>[2x]MLI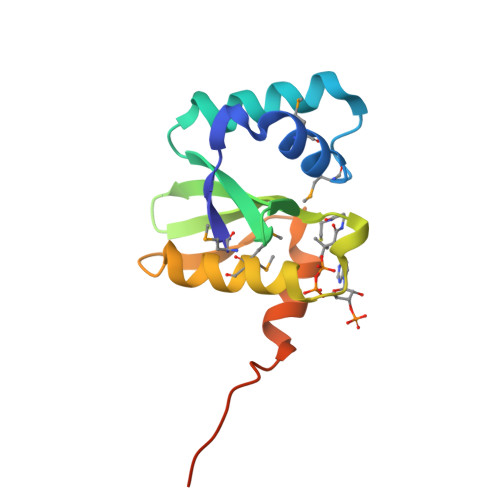RYKKSFEKIAMGLLSFMPNEKDLKQLQQTIKDYETDTDRQLFLWKEDEDIVGAIGVEKKDSEVEIRHISVNPSHRHQGIGKQMMDALKHLFKTQVLVPNELTQSFFERCQGQQDQDISYNNLEHHHHHH> ERAGPVTWVMMIACVVVFIAMQILGDQEVMLWLAWPFDPTLKFEFWRYFTHALMHFSLMHILFNLLWWWYLGGAVEKRLGSGKLIVITLISALLSGYVQQKFSGPWFGGLSGVVYALMGYVWLRGERDPQSGIYLQRGLIIFALIWIVAGWFDLFGMSMANGAHIAGLAVGLAMAFVDSLN

Rhomboid intramembrane proteases are evolutionarily conserved proteins with numerous important biological functions, including growth factor secretion, regulation of mitochondrial dynamics, and membrane protein quality control (Fleig et al., 2012). Rhomboids are serine proteases with a Ser-His catalytic dyad (Wang et al., 2006), and they recognize their transmembrane substrates in a two-tier process. It is assumed that first a portion of the transmembrane domain of the substrate docks into an intramembrane interaction site of rhomboid within the plane of the lipid bilayer, upon which a linear segment of the substrate (possibly generated by local unfolding of the top of the substrate's transmembrane helix) interacts with the water-exposed active site (reviewed in Strisovsky, 2016a, Strisovsky, 2013).

To gain insight into these preferences and their possible interactions, we have generated tetra- and pentapeptidyl chloromethylketones (CMK or cmk henceforth) harboring amino acids preferred in positions P5 to P1 by the Escherichia coli rhomboid GlpG (GlpG henceforth), using the sequence background of the Providencia TatA (Stevenson et al., 2007), represented by the parent compound Ac-IATA-cmk. To provide mechanistic explanation for the observed increase in inhibitory potency, we determined the structures of GlpG in complex with Ac-RVRHA-cmk and Ac-VRHA-cmk. The side chain of Arg in the P5 position of Ac-RVRHA-cmk could not be modeled due to poor electron density, and the two structures are otherwise virtually identical; superposition of all corresponding Cα atoms yields a root-mean-square deviation of 0.19 Å per atom (using the SSM method as implemented in CCP4MG v2.10.4; Krissinel and Henrick, 2004, Mitchell et al., 1990). Both inhibitors interact with the L3 and L5 loops via main-chain hydrogen bonds, and via hydrogen bonds involving the side chains of the strongly preferred Arg and His in the P3 and P2 position, respectively. The interactions of the residues in the P4, P3, and P2 positions with the enzyme are structurally independent, explaining why the effects of substitutions in these positions are additive. The overall binding mode of both compounds into the rhomboid active site is similar to the binding mode of peptide aldehyde Ac-VRMA-cho (Cho et al., 2016). Collectively, these data show that rhomboid subsite preferences are additive in the context of an active site targeted inhibitor and that sequence optimization in this region can significantly increase the inhibitory potency of the compounds.> EAEATQACLPVGSRKNGMNVNFYKYSLQDSTTYSDPQYMAYKYSDTKKLGSVSGQTHLSIYYGPNTAFWNTASWSSDLF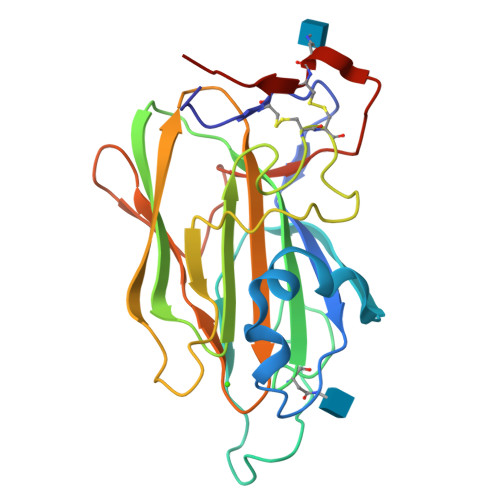GFYTTPTNVTVEMTGYFLPPQTGSYTFKFATVDDSAILSVGGSIAFECCAQEQPPITSTDFTINGIKPWDAAAPTDIKGSTYMYAGYYYPIKIVYSNAKALARLPVSVVLPDGTEVNDDFEGYVYSFDDDLSQSNCTIPDPSKHT>QQQHKV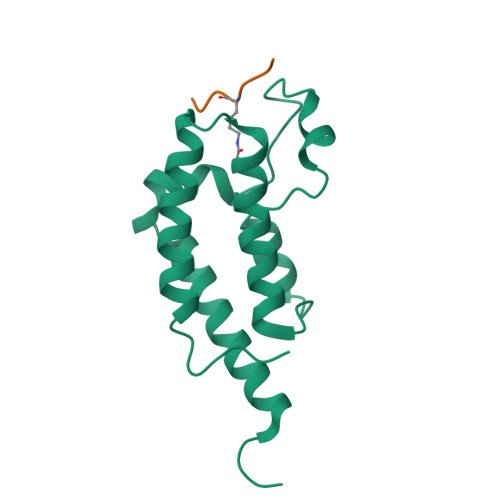LKTVKVTEQLKHCSEILKEMLAKKHLPYAWPFYNPVDADALGLHNYYDVVKNPMDLGTIKGKMDNQEYKDAYEFAADVRLMFMNCYKYNPPDHEVVAMARTLQDVFELHFAKIPDEPIES[2x];>[2x]KAPRKQLATK(2R,4S)-5,5-dimethyl-2-{(1R)-2-oxo-1-[(phenoxyacetyl)amino]ethyl}-1,3-thiazolidine-4-carboxylic 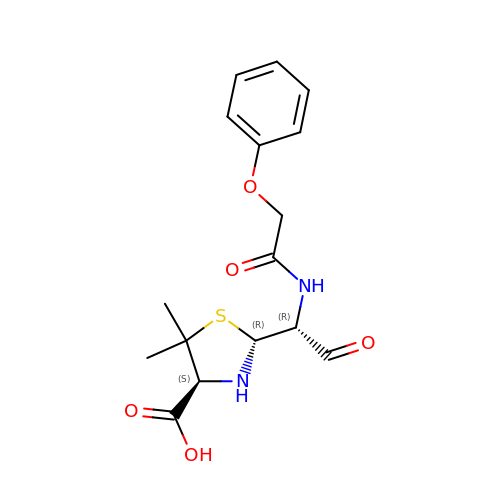acid | C16 H20 N2 O5 S | OQVOJWZOUWGSDX-KWCYVHTRSA-N(3R,4S)-1-[(4-amino-5H-pyrrolo[3,2-d]pyrimidin-7-yl)methyl]-4-[(hexylsulfanyl)methyl]pyrrolidin-3-ol 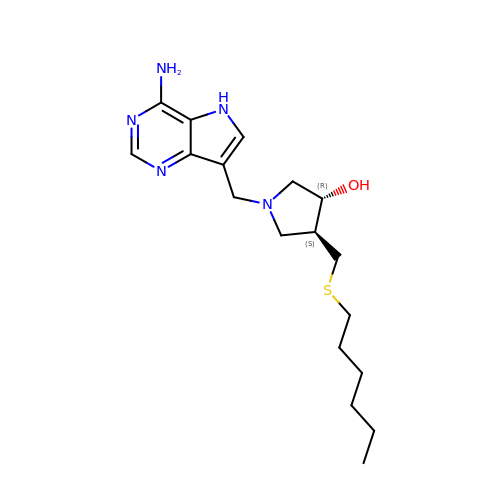| C18 H29 N5 O S | HXJWTLYUDABXFG-CABCVRRESA-N The type VI secretion system (T6SS) is a molecular machine utilised by many Gram-negative bacteria to deliver antibacterial toxins into adjacent cells. Here we present the structure of Tse15, a T6SS Rhs effector from the nosocomial pathogen Acinetobacter baumannii. Tse15 forms a triple layered β-cocoon Rhs domain with an N-terminal α-helical clade domain and an unfolded C-terminal toxin domain inside the Rhs cage. Tse15 is cleaved into three domains, through independent auto-cleavage events involving aspartyl protease activity for toxin self-cleavage and a nucleophilic glutamic acid for N-terminal clade cleavage.

Single particle cryo-electron microscopy (cryoEM) of the purified wildtype Tse15 revealed two major 3D particle classes; both monomeric in assembly but one that resembled the expected β-cocoon of the Rhs domain and a second that had the Rhs domain with a globular protrusion at one end (purple and yellow respectively). A map of Tse15 was produced with the clade domain present at a maximum resolution of 3.08 Å. Following refinement and manual adjustments, the final model of Tse15 spanning residues 14–1395 was produced that resolved the structure of an α-helical clade domain (residues 14-333) and a core β-strand rich cage (residues 335–1395) (in orange and grey respectively). We could resolve the cleavage point between the N-terminal clade and Rhs domains, with the sequence matching the previously identified cleavage site and a clear break in the connective density of the polypeptide chain. The toxin density could be observed lining the interior wall of the β−stranded cage and appeared to have elements of secondary structure but not an overall globular fold. Between the Rhs and the toxin, there is a clear break in connective density that corresponds to the cleavage site of the toxin as determined by N-terminal sequencing (L1395). We were able to de novo build four separate peptides (chains B, C, D and E) into regions of convincing density, placing a total of 106 of the 195 residue CTD toxin (blue). These chains were modelled as poly-alanine with some glycine residues placed to allow an improved fit to the density. We also noted that the short helical chain C (10 residues) was localised to the exterior cleft of the Rhs domain, suggesting that this is indeed the point of toxin entrance or exit (blue). Also localised close to the entrance and chain C was the longer chain E (43 residues) that appeared to interact with the end of the clade domain, close to the cleavage site.

> MAWSHPQFEKSAAKENTQQKEIKRQPAVELAVFNLNSVTDVADLQMIASQVQLYLQVCGNTTLEQIKSKANITTVANIFALTGSVLDLMLYATDKKTGDAAVQRGALLAANLIGLFSEPNNEAHARMALRPMFGLMAECLYRENGKIKETDIKRLGLHLNAMIAGDLENFLKETQAKLSSLLISATTLGVTILQSMATPATGINAGITTAAGASAEKRDPKLKFTNWAVPLIDLLGKPSQANLTPKIQPNITSRLQQEATQAIAALSQTLQQQANAGQKYTLAWLLQETLKAIQALENKGNASVPINQTGEYERHTKGDTLEFVSLQADALNAPPCEGADSQSGKSISYSIGAERVQHADFYLPKIGFSFIRQYNSQMDEFDQSMVGARWMMPFSNMIQQNAQGYLFIDSKGRKHQLPVSIIFETYEVPYEGWIIKPLKNGELILDFGGEWRSHFQSFDGGKNYYLVKKMNETSQEEILLEYLLLDHIAYLKVINFKLKQAEYELKFAFNEQVKIIAVFLDDKAEPLARYEYDTQGNLIKAIDQNGHTRTYEYNQFHQLTRYTDRTGRGQNIRYESTEAKAKAIEEWADDGSFHTKLKWHPRLRQVAVYDAYDVPTYYYFDLDGFTYRTRLADGRESWYSRDGKKRITRQIDFDGRETQQEYNDQDQLVKIVQPNGGIIRFAYNKQGNLVEIKDPEGSIWKREYDENRNVSKEINPLGHITQYKYNNDNQLVEVIDAKGGVKKIQYNELGQMISYTDCSGKSSTWEYDEDGALTAEQTANNKVVQYFYSTKGRDKGQLQSIIYPDGLKEYFEHDEEGRLLKHTDTKGLVTEYKYNQVGLLEQRIDANRHSVAYQWDKQGRIQKLINQNQAEYLFGYNPYGYLIREQAFDGEEKHYSYNENGRLFQIRRPNILTQFDYYADGQIASKSFTHLHTGQKQTEQFDYNLNSQLSRASNEVSQIDLYRNALGQLVREHQHYKIPELKPLTAVLHYEYDELGNLIKTIRPDGHTLNHLVYGSGHIYAIGLNNQEVVSFQRDDLHRETTRLLANGLMQTKQYNDVGLLSSQFIQPEQETQDYLQYQAHRKYHYDKNYLLSQVEDSRLGKLNYQYDPIGRLIAAQSLHKTESFNFDPAGNLIDSESVLSPAQIKNNLIKSYKGKHYQYDVQGNVTEIIQAGKNLKLTWDNQNRLIRSDNNGLVTEYGYDVFGRRLYKKTAKELTLFGWDGDLMIWESFKSAQTNYTKHYIYEPDSFVPLLQAGYKDFIQLIETPDYQEYQTKPYSIYKDPVWNRNLGKERTALEQFTFYHCDQVGTPQTMTNIRGECVWEILQDTWGAVSQIKALNQDNPFEQNNLRFQGQYYDRETELHYNRYRYYEPHSARYVSKDPIGLEGGMNTSSYVSDPNQWIDPKGLNSFNYGEMFGIPASAQSGLAYQGQRNYECYAETGELCKIKVPPLFDYVACSGGGLGIGVGFVKNQWTGEYYISGSKDSLLIPVAKSVAQNKQFSAKDLAGASCVGGNIHNIPSYTKTTMTMGEITNEFVSGASVTVGGGAYGAVANVVVPLVSKSSPVKGTWASELGVGTPGFNVGVSGTVSVDTILDAVKPSKKHHHHHH(2S)-piperidine-2-carboxylic acid | C6 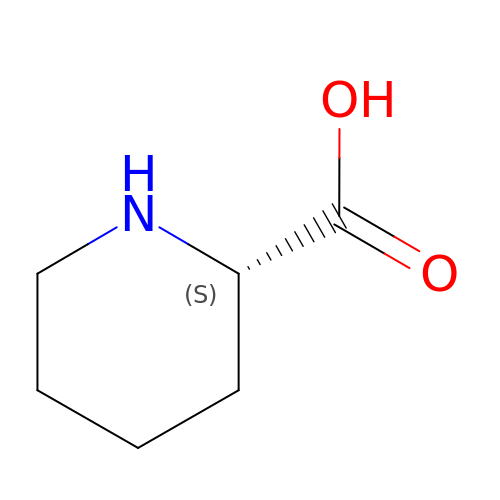H11 N O2 | HXEACLLIILLPRG-YFKPBYRVSA-N> MEPRTIACPHKGCTKMFRDNSAMRKHLHTHGPRVHVCAECGKAFVESSKLKRHQLVHTGEKPFQCTFEGCGKRFSLDFNLRTHVRIHTGDRPYVCPFDGCNKKFAQSTNLKS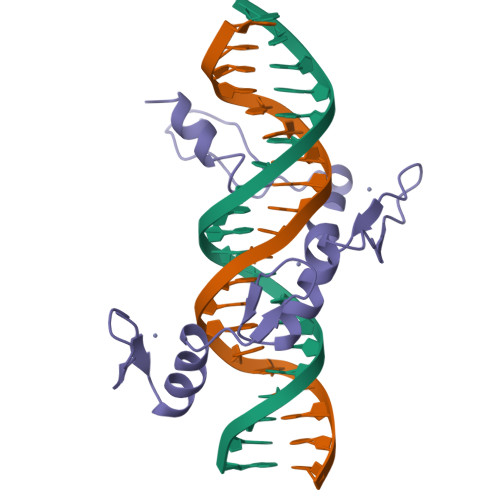HILTHAKAKNNQ>[2x]HHHHHHHHGSGAGWSHPQFEKGGSGLVPRGSGSVPAGAKCRLVETLPENMDFRSDHLTTFECFNEIITLAKKYIYIASFCCNPLSTTRGALIFDKLKEASEKGIKIIVLLDERGKRNLGELQSHCPDINFITVNIDKKNNVGLLLGCFWVSDDERCYVGNASFTGGSIHTIKTLGVYSDYPPLATDLRRRFDTFKAFNSAKNSAANLASAAAALPVSTAYHIKNPIGGVFFTDSPEHLLGYSRDLDTDVVIDKLKSAKTSIDIEHLAIVPTTRVDGNSYYWPDIYNSIIEAAINRGVKIRLLVGNWDKNDVYSMATARSLDALCVQNDLSVKVFTIQNNTKLLIVDDEYVHITSANFDGTHYQNHGFVSFNSIDKQLVSEAKKIFERDWVSSHSKSLKI

F13 is a phospholipase anchored to membranes via two palmitoylated cysteines located in a hydrophobic membrane-interacting region (MIR). Tecovirimat is an inhibitor of mature virus wrapping widely used to treat mpox patients infected with clade IIb strains. Tecovirimat binding to F13 blocks viral wrapping, but the structural mechanism is poorly understood. We showed that F13 forms a homodimer on membranes, and tecovirimat inserts into a cavity formed between the two protomers.

For the structural studies, we produced a soluble variant of F13 (sF13) by removing the hydrophobic N-terminal tail (amino acids 2–5) and by introducing five mutations in the MIR. We obtained two different crystal forms. In both, sF13 featured a homodimer stabilized by two helices and a β-hairpin with an interface area of 939 Å2, formed by a network of hydrogen bonds involving residues Y253, N259, N267, Y285, S292 and N300. The contact region forms a large cavity of 290 Å3. The hydrophobic N termini and MIRs were located on one side of the dimer, and the two phospholipase D (PLD) catalytic pockets were pointed outwards. Here we report the structure of an F13 homodimer using X-ray crystallography, both alone (2.1 Å) and in complex with tecovirimat (2.6 Å). Structural analysis revealed a large cavity at F13’s dimerization interface, which is absent in PLD3 and PLD4 homodimers. We hypothesized that this cavity reduces the stability of the F13 dimer.>AEGTRGRSSTARCSLFGSDFVNTFDGSMYSFAGYCSYLLAGGCQKRSFSIIGDFQNGKRVSLSVYLGEFFDIHLFVNGTVTQGDQRVSMPYASKGLYLETEAGYYKLSGEAYGFVARIDGSGNFQVLLSDRYFNKTCGLCGNFNIFAEDDFMTQEGTLTSDPYDFANSWALSSGEQWCERASPPSSSCNISSGEMQKGLWEQCQLLKSTSVFARCHPLVDPEPFVALCEKTLCECAGGLECACPALLEYARTCAQEGMVLYGWTDHSACSPVCPAGMEYRQCVSPCARTCQSLHINEMCQERCVDGCSCPEGQLLDEGLCVESTECPCVHSGKRYPPGTSLSRDCNTCICRNSQWICSNEECPGECLVTGQSHFKSFDNRYFTFSGICQYLLARDCQDHSFSIVIETVQCADDRDAVCTRSVTVRLPGLHNSLVKLKHGAGVAMDGQDVQLPLLKGDLRIQHTVTASVRLSYGEDLQMDWDGRGRLLVKLSPVYAGKTCGLCGNYNGNQGDDFLTPSGLAEPRVEDFGNAWKLHGDCQDLQKQHSDPCALNPRMTRFSEEACAVLTSPTFEACHRAVSPLPYLRNCRYDVCSCSDGRECLCGALASYAAACAGRGVRVAWREPGRCELNCPKGQVYLQCGTPCNLTCRSLSYPDEECNEACLEGCFCPPGLYMDERGDCVPKAQCPCYYDGEIFQPEDIFSDHHTMCYCEDGFMHCTMSGVPGSLLPDAVLSSPLSHRSKR[16x];>SLSCRPPMVKLVCPADNLRAEGLECTKTCQNYDLECMSMGCVSGCLCPPGMVRHENRCVALERCPCFHQGKEYAPGETVKIGCNTCVCQDRKWNCTDHVCDATCSTIGMAHYLTFDGLKYLFPGECQYVLVQDYCGSNPGTFRILVGNKGCSHPSVKCKKRVTILVEGGEIELFDGEVNVKRPMKDETHFEVVESGRYIILLLGKALSVVWDRHLSISVVLKQTYQEKVCGLCGNFDGIQNNDLTSSNLQVEEDPVDFGNSWKVSSQCADTRKVPLDSSPATCHNNIMKQTMVDSSCRILTSDVFQDCNKLVDPEPYLDVCIYDTCSCESIGDCACFCDTIAAYAHVCAQHGKVVTWRTATLCPQSCEERNLRENGYECEWRYNSCAPACQVTCQHPEPLACPVQCVEGCHAH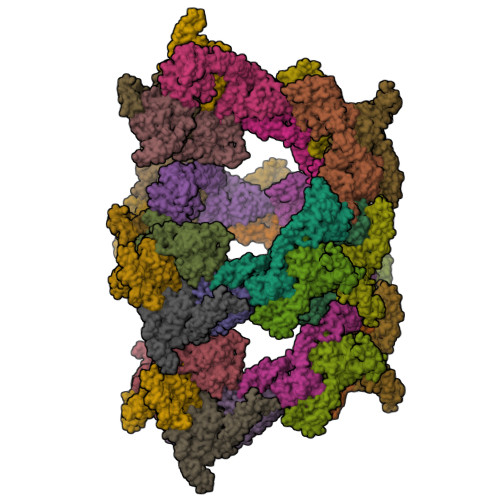CPPGKILDELLQTCVDPEDCPVCEVAGRRFASGKKVTLNPSDPEHCQICHCDVVNLTCEACQEPGGLVVPPHHHHHH[16x]> MQ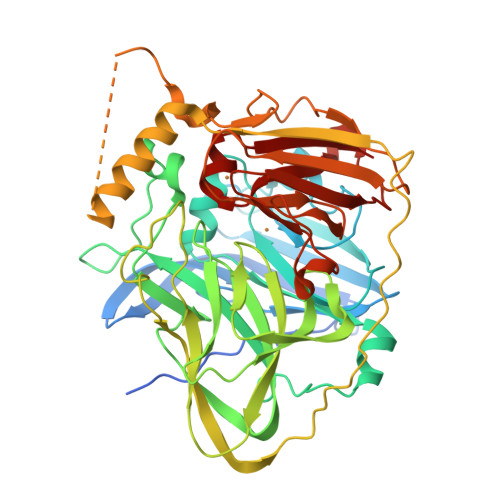RRDFLKYSVALGVASALPLWSRAVFAAERPTLPIPDLLTTDARNRIQLTIGAGQSTFGGKTATTWGYNGNLLGPAVKLQRGKAVTVDIYNQLTEETTLHWHGLEVPGEVDGGPQGIIPPGGKRSVTLNVDQPAATCWFHPHQHGKTGRQVAMGLAGLVVIEDDEILKLMLPKQWGIDDVPVIVQDKKFSADGQIDYQLDVMTAAVGWFGDTLLTNGAIYPQHAAPRGWLRLRLLNGCNARSLNFATSDNRPLYVIASDGGLLPEPVKVSELPVLMGERFEVLVEVNDNKPFDLVTLPVSQMKMAIAPFDKPHPVMRIQPIAISASGALPDTLSSLPALPSLEGLTVRKLQLSMDPMLDMMGMQMLMEKYGDQAMAGMDHSQMMGHMGHGNMNHMNHGGKFDFHHANKINGQAFDMNKPMFAAAKGQYERWVISGVGDMMLHPFHIHGTQFRILSENGKPPAAHRAGWKDTVKVEGNVSEVLVKFNHDAPKEHAYMAHCHLLEHEDTGMMLGFTV> MRNDGGFLLWWDGLRSEMQPIHDSQGVFAVLEKEVRRLGFDYYAYGVRHTIPFTRPKTEVHGTYPKAWLERYQMQNYGAVDPAILNGLRSSEMVVWSDSLFDQSRMLWNEARDWGLCVGATLPIRAPNNLLSVLSVARDQQNISSFEREEIRLRLRCMIELLTQKLTDLEHPMLMSNPVCLSHREREILQWTADGKSSGEIAIILSISESTVNFHHKNIQKKFDAPN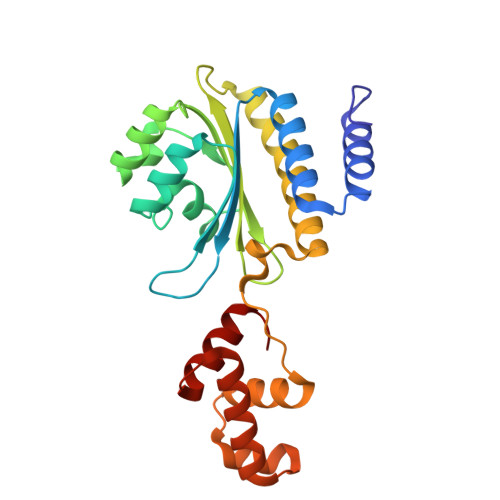KTLAAAYAAALGLI> MPSKPLRPCNKIGCTNLTRDRYCEQHKHLAEQRQRTRRNDKEYDKHKRNQQARAFYHSREWERTRLAVLAKDNYLCQHCLKEKKITRAVIVDHITPLLVDWSKRLDMDNLQSLCQACHNRKTAEDKRRYG

An HNH endonuclease from the thermophilic bacteriophage GVE2, a thermophilic and lytic bacteriophage that infects Geobacillus sp. E263 isolated from a deep-sea hydrothermal field in the east Pacific1920, was the first thermostable member of HNH endonucleases from thermophilic bacteriophages to be biochemically characterized. The overall structure of GVE2 HNHE contains two antiparallel β-sheets and four α-helices, and shares a conserved ββα-metal fold with those of other HNH endonucleases. Sequence analysis shows that residues H93, N109 and H118 in GVE2 HNHE are the key residues in the conserved ββα-metal fold motif, and could be components of the active site of the enzyme. Residues H93, N109 and H118 in GVE2 HNHE are key amino acid residues for DNA nicking.

Note that we solved the crystal structure of the truncated GVE2 HNHE from N39 to G130. The initial 38 residues (M1-R38) could not be solved because of the disordered electron density, indicating the N-terminal region of the protein is very flexible. Like other endonucleases, a zinc ion exists in the center of the structure of GVE2 HNHE and is coordinated by Cys76 (in the short loop linking helix α2 and α3), Cys79 (in the helix α3), Cys114 (in the short loop linking the helix α4 and β2), and Cys117 (in the helix α4 at the end of the C-terminal domain). It resembles the Zn2+-bound structure of Gme HNHE11, suggesting that the Zn-finger domain in HNH endonuclease is conserved. Firstly, GVE2 HNHE possesses an extra α-helix (α3: residues 85–92) at the C-terminus, which is absent in Gme HNHE. However, no additional metal ion was observed in the HNH motif of GVE2 HNHE. Here, we found that GVE2 HNHE and the Zn ion were co-crystalized, supporting the importance of the Zn ion for DNA nicking. There is no significant structural change for the two structures of GVE2 HNHE with Mn2+ and Zn2+, however, the C-terminus of GVE2 HNHE shifts by a distance of approximately 1.3 Å upon binding of Mn2+.>MNFNVGVDFPSFIAWDGTTSFPVKIDGFNQFGFTFKVIEELTADVPFNIFYHEASEADPCVPGPAIRVPDVPFCDGVATADGLATVVIPEAVAVDSFCAGSVPCFNGPWISIAPVTVNADSAKVQVTVTMKGATR[30x];>[17x]MANKESEQNGLEAISGDIEKLSSNVDLFSKAMDDKYKELTARFDGQKSDSEEIRKAAEQATKEYAELSAKHQFFTEELVAMKARLDSPIMRSQADLDDHDRKTAIQLQRNMHEFRGGDPKEFVADESNLVDLKAYRSAVRKMLKVGIESKERVISSMTDVERKAFEASTIGPAFFTPQVLALEVDCNIECASLLDLYGQIEVSRSTFTYMKIADYGQLGEYTCDAKCDAEFGEPGNIRHLEGKTYDYRGVFCFNRKNLQEANYDFLSFMIGAAQRSHRINRNRALMVGDGINEPKGWLKEDCFPTFLTLPVNTGTPENPVQTPAFLAQDWRRFVTSFPAEYGDARSVMHQNVFGYLAAMVDANGRFLFGDGDLTFSPDLVRERIRISNCLPDPTEGNTKGGTGQDAFAAGSFIAAQAAWKTAYYAVEKRPMFFEQYEGGSSAWCVKYQFGAEDGGFVGCCEHGRVLRIG;>MVSLDCRNTCAPAPASRLVQPPCFVCRDVFPLPVAPNPPGPVSAIIGTTPSTFSLKPDGTFITGTG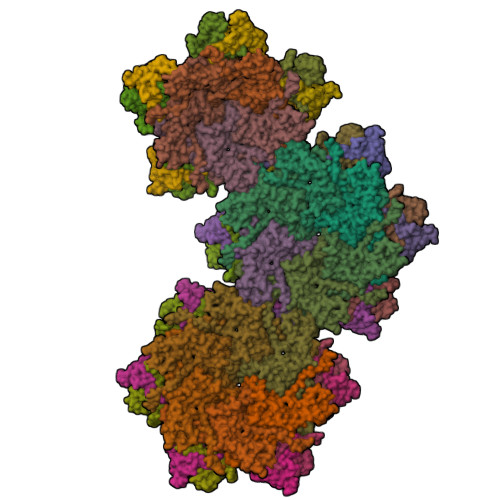ISSSGSAVATDGSLELFLAPLVAHVTGSEMSPPYAVELQEGQELAIVFGATLKSGFGVRITDYYDVVFNIVSSEGTKQLKLVPGNTPSGYIWTDGEGYNIVDSNGDFHSVQNVTRPSFLGITDTGVLWQLVGYLKGTTQAELAIAIEVTVTHAN[5x];>[12x]MIKLNCRPLCQTPTASRLVSPPCFICRR> SESSIVNACLRYLGYSKSMCHEKMPIFMDIAFIEYCFNLSLDPSSFQGGASQQILWEYSLISNALERLENIELERQNCMREDGLSKYTNSLLLNKETLNNEALKLYSCAKAGICRWMAFHFLEQEPIDHINFTKFLQDWGSHNEKEMEALQRLSKHKIRKRLIYVSQHKKKMPWSKFNSVLSRYIQCTKLQLE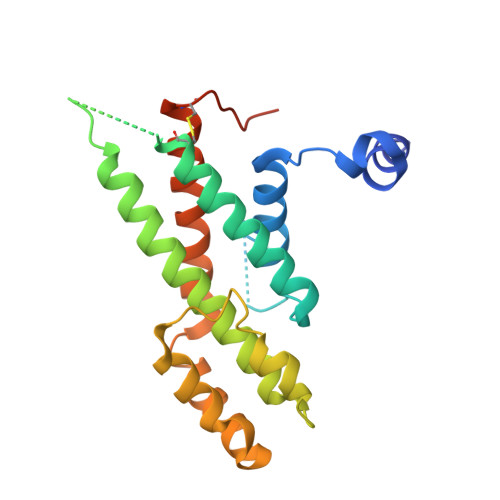VFCDYDFKQREIVKMLTSNIN2-({[(2R,4S)-2-[2-(4-chlorophenyl)ethyl]-2-(1H-imidazol-1-ylmethyl)-1,3-dioxolan-4-yl]methyl}sulfanyl)-5-(trifluoromethyl)pyridine | 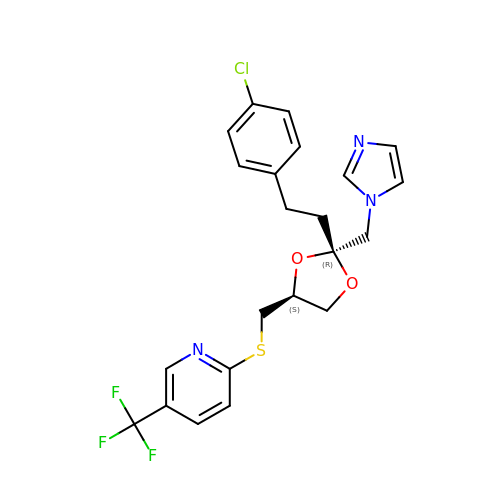C22 H21 Cl F3 N3 O2 S | QJIXKBNNYAEGKH-PZJWPPBQSA-N3,5-dimethyl-N-{2-[4-(4-methylbenzyl)piperidin-1-yl]-3,4-dioxocyclobut-1-en-1-yl}-1,2-oxazole-4-sulfonamide 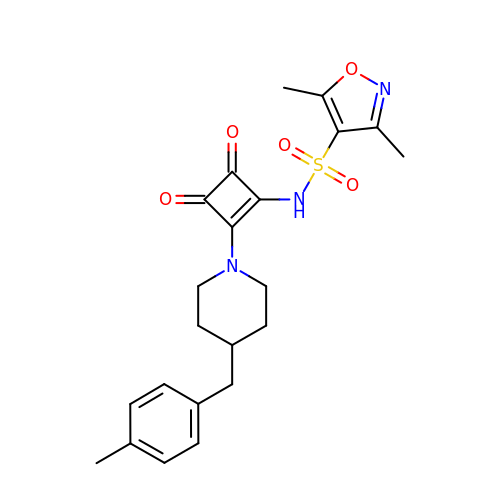| C22 H25 N3 O5 S | DJQHTHRCUXNHLQ-UHFFFAOYSA-N> GPHMGLQESFGVAAEDKIFGGSGSFIPRCMEAMKGVRSMLQCMADKANARNMLQQASLVRPLDNQETLDFSRLSLVEQHECLASILHAAVQRHHATIADFQDFIKILRKWDKYDHFLIHLIPVLAAYITEFGSPEGMGDLQQARRLNDFICKGGDEDSWALPVLGAAVRAWWIAEHNGFYLDDTVQDLRGINLDEEDEQRTKQFLDALKEGAFDFILSVAADCKAQEWQDPSQLGARQWLQRKIPSLPSEPFPFSHFLQHSLMVHLEGFVDATISNLPDVLRKLRTEEDEQRQLRPNHEQDMDLERFLIIISYAYEGRPDAAMSFWEDPDSNLAGFLQWASRRASTPLVSAFCEMLRCLADNEECATAAHNFLLDEGHQASGKMKRSQSLTWSQIFKELEYFTTKVCSERPNPPQASMHRPGRPGADPAEIEPESALMLECYLRLIAKLATESEIARKRLIMDEDFNLVDTILKLSVGVIPHRLRACIFYVLKALMIRKTHEELDAMWRWVEAWMTNPFSSLPGSQGAPQRISFLGQTPGPQECMEMMFREFGTGFEQSNAFIQLLTTLLVPPEGLNSLNDSVPFPEWLGSSIRTLGIEPYVDFVFDVFANRTKDISDPSQLRILRLSCLDFVMVCLVTFNEDLIVLGHESNISIDDAMAATNLATYVRLHPFSRVMEWLFNEKVITSLINTIHQDPISLGSASPDSPLVVS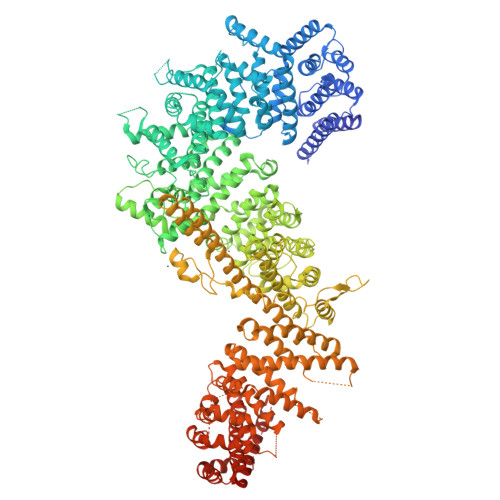ILRAIQVMIKALELQETYLHLVRPEVLRYQGEAGVRRKPVANAAYSAFEDGILSHLSLVVDLGKYCNLGHAELTLACLKLLEKISTSSRILSAWSPDSGRLGHRNKAIVQLERNGEGETISASLSASIMATLDPALAASGENYRVKLAILDFLYACLRATPDQPTIAHQLLGFHCELSKLGIEPKGPFDMQKSLFHSLLNVLITLTVSEEEQGMRGYLVTLKYRVLRILQLLWKSPLSASLVMDELRATNFLFHMLLREVQIQPQLPWDGQLVTGCEFLLSDASLAYIDYLASRAAIFEYIGKELCSVSQNRIPSIKRQIFDALNGQIFVDEEAPLTIPSIFDFFDFINTDYKWEEIPSPHFTYLKDLDLGPCILEHKYAGVHYDIRKAQEILALKRKEYEHSQLATPEFLETVELEEKVLIEWLTVRNRANLLLTARLNLLQAWANLLLVMIESNDFKSTPKMAFLLQALQAILPTLEAFSSLKSDEAFELARVAKVLLWKLDFSQDSDAGLDREQFTVGNLIGDKLFQLFQLCLSAISQCSGTPELRSLYYSICYRYLTAVVDNDATVAATPASSTIGPTRSVTNARARTLKAITLYGDRLLNVICDDAYGSDTTCQTAAMILLNALVHTSRASSAAGVSPADVDCPIIDALNRLNFIGVLVDSLKEILNEWLAPSSTFDPSLSTNASPSLPIPASPSQQYTSAKLALLLQLCQTRQGAKYVLQANLFRALEQSGVFAADPELVEVDSESGVPRVVALERHYALLVALARVVGAAVTARGAHNIVQGRKFLTQHRGLVVHVLKKNAGIGGGVVGNSLASSINGGSTATMTRRDEILAQQALEERIEELAEAFMLLITATGFLEYESEQVPSEQPRAHTTFFH> GSTSSVQRDDFHWEEYLKETGSISAPSECFRQSQIPPVNDFKVGMKLEARDPRNATSVCIATVIGITGARLRLRLDGSDNRNDFWRLVDSPDIQPVGTCEKEGDLLQPPLGYQMNTSSWPMFLLETLNGSEMASATLFKKEPPKPPLNNFKVGMKLEAIDKKNP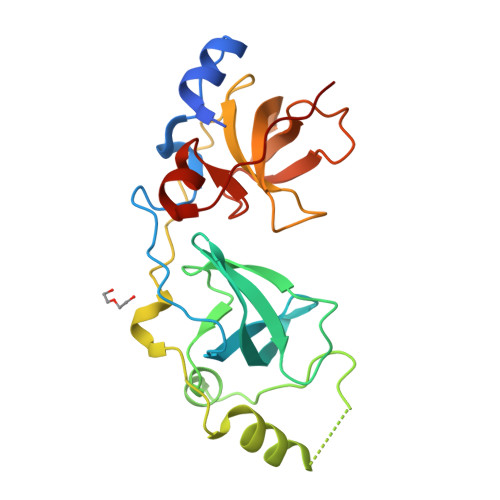YLICPATIGDVKGDEVHITFDGWSGAFDYWCKYDSRDIFPAGWCRLTGDVLQPPGTS>MANNSFITLNPSLPNSENSVIEAFSYKCIHCYNHHKFGTLEKLREAFPNLHFKLYPVSLMNGEFSKEMNELFAFAQYKDEQNGKDASYSDSLSHKLADVYFVSYFLNKQRNFSNLDEFYDIGLKAMNVNKNEVLNFLNTPKAKEILSEFQRANDIAKTYGTPAFVVNGKYQINPSAINSMQDLEDLVKKLSNMKLEHHHHHH[2x]

The bacterial proteins of the Dsb family catalyze the formation of disulfide bridges between cysteine residues that stabilize protein structures and ensure their proper functioning. The oxidative part of this network consists of two monomeric DsbAs (DsbA1 and DsbA2) related to EcDsbL, which cooperate with one DsbB. The solved structures of both CjDsbAs, especially the length and amino acid sequences of their L2 and L3 loops that are essential elements of the monomeric thiol oxidoreductases, were different from that of EcDsbA but similar, though not identical, to that of EcDsbL, which affected their functioning.

CjDsbA1 crystallized in the C2 and P212121 space group containing two monomers in the ASU for the monoclinic form and one molecule per ASU for the orthorhombic form, while CjDsbA2 crystallized in P3221 with a single chain in the ASU. In the monoclinic CjDsbA1, the C-terminal HisTag as well as 3–4 N-terminal residues could not be modelled, and in chain B, two residues (108–109) on the surface could not be modelled. The superposition of monoclinic and orthorhombic forms of CjDsbA1 showed relatively small differences between them, which was confirmed by an RMSD value of 0.45 Å. The active site of CjDsbA1 was observed in the reduced form, while the CjDsbA2 formed a clear disulfide bond. This was due to differences in protein purification procedures. CjDsbA1 was purified under reducing conditions. It should be noted that the CjDsbA1 redox potential was the highest among the characterized DsbAs so far described; EcDsbL has a redox potential of −95 mV and N. meningitidis lipoprotein NmDsbA2 has a redox potential of −79 mV. Previously, we found that CjDsbA1 present in wild-type (wt) cells was present in its oxidized form, but it was mainly present in its reduced form in cells lacking CjDsbB; also, the lack of CjDsbA2 had no impact on its redox state. We documented that CjDsbA1 complemented the lack of the EcDsbA in the motility test, in contrast to CjDsbA2, which was inactive in this assay. First of all, in E. coli JCB817, CjDsbA1 formed higher molecular weight oligomeric complexes (~46 kDa), which disappeared when cells were treated with the reducing agent DTT; in E. coli JCB818 lacking EcDsbB, these complexes migrated slower when compared to their mobility in E. coli JCB817.> MSEIGTGFPFDPHYVEVLGERMHYVDVGPRDGTPVLFLHGNPTSSYLWRNIIPHVAPSHRCIAPDLIGMGKSDKPDLDYFFDDHVRYLDAFIEALGLEEVVLVIHDWGSALGFHWAKRNPERVKGIACMEFIRPIPTWDEWPEFARETFQAFRTADVGRELIIDQNAFIEGALPKYVVRPLTEVEMDHYREPFLKPVDREPLWRFPNELPIAGEPANIVALVEAYMNWLHQSPVPKLLFWGTPGVLIPPAEAARLAESLPNCKTVDIGPGLHYLQEDNPDLIGSEIARWLPALHHHHH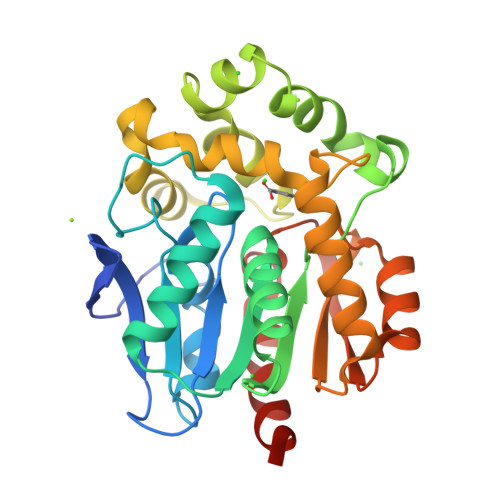H>MAEKQKHDGRVKIGHYVLGDTLGVGTFGKVKIGEHQLTGHKVAVKILNRQKIRSLDVVGKIKREIQNLKLFRHPHIIKLYQVISTPTDFFMVMEYVSGGELFDYICKHGRVEEMEARRLFQQILSAVDYCHRHMVVHRDLKPENVLLDAHMNAKIADFGLSNMMSDGEFLRTSCGSP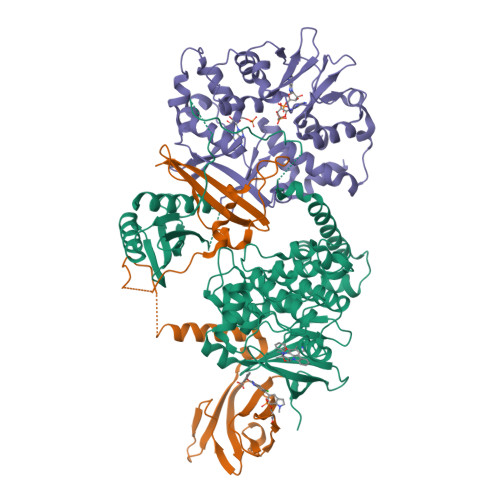NYAAPEVISGRLYAGPEVDIWSCGVILYALLCGTLPFDDEHVPTLFKKIRGGVFYIPEYLNRSVATLLMHMLQVDPLKRATIKDIREHEWFKQDLPSYLFPEDPSYDANVIDDEAVKEVCEKFECTESEVMNSLYSGDPQDQLAVAYHLIIDNRRIMNQASEFYLASSPPSGSFMDDSAMHIPPGLKPHPERMPPLIADSPKARCPLDALNTTKPKSLAVKKAKWHLGIRSQSKPYDIMAEVYRAMKQLDFEWKVVNAYHLRVRRKNPVTGNYVKMSLQLYLVDNRSYLLDFKSIDDEVVEQRSGSSTPQRSCSAAGLHRPRSSFDSTTAESHSLSGSLTGSLTGSTLSSVSPRLGSHTMDFFEMCASLITTLAR[2x];>[2x]MGLNDIFEAQKIEWHEMGNTSSERAALERHGGHKTPRRDSSGGTKDGDRPKILMDSPEDADLFHSEEIKAPEKEEFLAWQHDLEVNDKAPAQARPTVFRWTGGGKEVYLSGSFNNWSKLPLTRSHNNFVAILDLPEGEHQYKFFVDGQWTHDPSEPIVTSQLGTVNNIIQVKKTDFEVFDALMVDSQKCSDVSELSSSPPGPYHQEPYVCKPEERFRAPPILPPHLLQVILNKDTGISCDPALLPEPNHVMLNHLYALSIKDGVMVLSATHRYKKKYVTTLLYKPI;>[2x]METVISSDSSPAVENEHPQETPESNNSVYTSFMKSHRCYDLIPTSSKLVVFDTSLQVKKAFFALVTNGVRAAPLWDSKKQSFVGMLTITDFINILHRYYKSALVQIYELEEHKIETWREVYLQDSFKPLVCISPNASLFDAVSSLIRNKIHRLPVIDPESGNTLYILTHKRILKFLKLFITEFPKPEFMSKSLEELQIGTYANIAMVRTTTPVYVALGIFVQHRVSALPVVDEKGRVVDIYSKFDVINLAAEKTYNNLDVSVTKALQHRSHYFEGVLKCYLHETLETIINRLVEAEVHRLVVVDENDVVKGIVSLSDILQALVLTGGEKKP> ETGRGCPTHCHCEPDGRMLLRVDCSDLGLSELPSNLSVFTSYLDLSMNNISQLLPNPLPSLRFLEELRLAGNALTYIPKGAFTGLYSLKVLMLQNNQLRHVPTEALQNLRSLQSLRLDANHISYVPPSCFSGLHSLRHLWLDDNALTEIPVQAFRSLSALQAMTLALNKIHHIPDYAFGNLSSLVVLHLHNNRIHSLGKKCFDGLHSLETLDLNYNNLDEFPTAIRTLSNLKELGFHSNNIRSIPEKAFVGNPSLITIHFYDNPIQFVGRSAFQHLPELRTLTLNGASQITEFPDLTGTANLESLTLTGAQISSLPQTVCNQLPNLQVLDLSYNLLEDLPSFSVCQKLQKIDLRHNEIYEIKVDTFQQLLSLRSLNLAWNKIAIIHPNAFSTLPSLIKLDLSSNLLSSFPITGLHG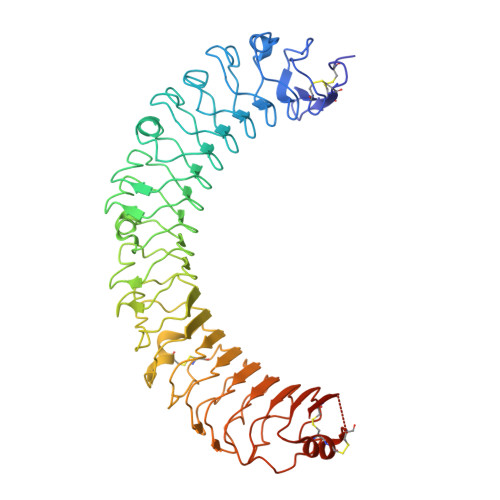LTHLKLTGNHALQSLISSENFPELKVIEMPYAYQCCAFGVCENNGNNGDSVQCSPSGTHHHHHHHHHH> MTSKETFTHYQPQGNSDPAHTATAPGGLSAKAPAMTPLMLDTSSRKLVA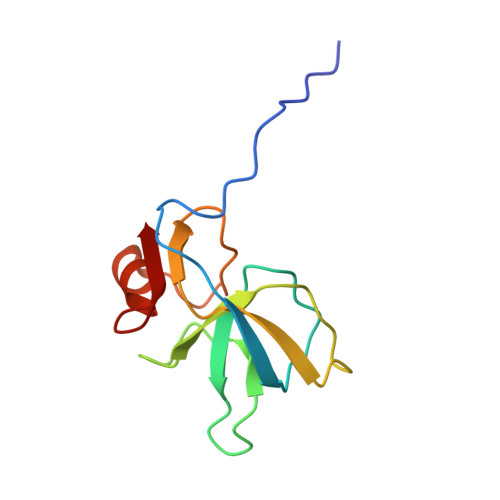WDGTTDGAAVGILAVAADQTSTTLTFYKSGTFRYEDVLWPEAASDETKKRTAFAGTAISIV>[2x]RAPAPATPHAPDHSPAPNSPTLTRPPEGP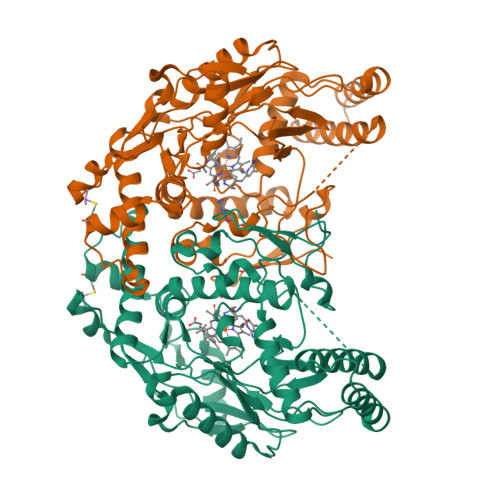KFPRVKNWELGSITYDTLCAQSQQDGPCTPRRCLGSLVLPRKLQTRPSPGPPPAEQLLSQARDFINQYYSSIKRSGSQAHEERLQEVEAEVASTGTYHLRESELVFGAKQAWRNAPRCVGRIQWGKLQVFDARDCSSAQEMFTYICNHIKYATNRGNLRSAITVFPQRAPGRGDFRIWNSQLVRYAGYRQQDGSVRGDPANVEITELCIQHGWTPGNGRFDVLPLLLQAPDEAPELFVLPPELVLEVPLEHPTLEWFAALGLRWYALPAVSNMLLEIGGLEFSAAPFSGWYMSTEIGTRNLCDPHRYNILEDVAVCMDLDTRTTSSLWKDKAAVEINLAVLHSFQLAKVTIVDHHAATVSFMKHLDNEQKARGGCPADWAWIVPPISGSLTPVFHQEMVNYILSPAFRAQPDPW> DGCYTWSGTLSEGSSGEAVRQLQIRVAGYPGTGAQLAIDGQFGPATKAAVQRFQSAY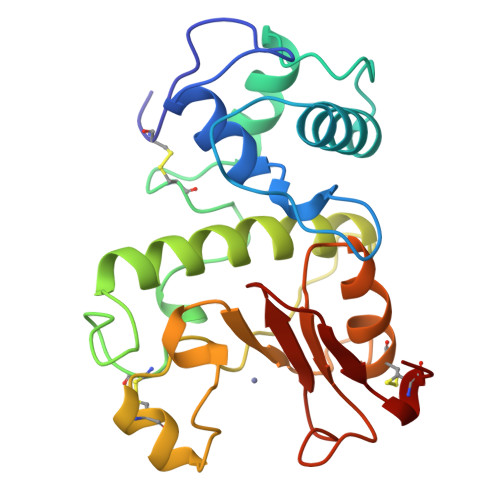GLAADGIAGPATFNKIYQLQDDDCTPVNFTYAELNRCNSDWSGGKVSAATARANALVTMWKLQAMRHAMGDKPITVNGGFRSVTCNSNVGGASNSRHMYGHAADLGAGSQGFCALAQAARNHGFTEILGPGYPGHNDHTHVAGGDGRFWSAPSCGI>MHHHHHHAAGIPMNNPAIKRIGNHITKSPEDKREYRGLELANGIKVLLISDPTTDKSSAALDVHIGSLSDPPNIAGLSHFLEHMLFLGTKKYPKENEYSQFLSEHAGSSNAFTSGEHTNYYFDVSHEHLEGALDRFAQFFLSPLFDESAKDREVNAVDSEHEKNVMNDAWRLFQLEKATGNPKHPFSKFGTGNKYTLETRPNQEGIDVRQELLKFHSAYYSSNLMAVVVLGRESLDDLTNLVVKLFSEVENKNVPLPEFPEHPFQEEHLKQLYKIVPIKDIRNLYVTFPIPDLQKYYKSNPGHYLGHLIGHEGPGSLLSELKSKGWVNTLVGGQKEGARGFMFFIINVDLTEEGLLHVEDIILHMFQYIQKLRAEGPQEWVFQELKDLNAVAFRFKDKERPRGYTSKIAGILHYYPLEEVLTAEYLLEEFRPDLIEMVLDKLRPENVRVAIVSKSFEGKTDRTEEWYGTQYKQEAIPDEVIKKWQNADLNGKFKLPTKNEFIPTNFEILPLEKEATPYPALIKDTAMSKLWFKQDDKFFLPKANLNFEFFSPFAYVDPLHSNMAYLYLELLKDSLNEYAYAAELAGLSYDLQNTIYGMYLSVKGYNDKQPILLKKIIEKMATFEIDEKRFEIIKEAYMRSLNNFRAEQPHQHAMYYLRLLMTEVAWTKDELKEALDDV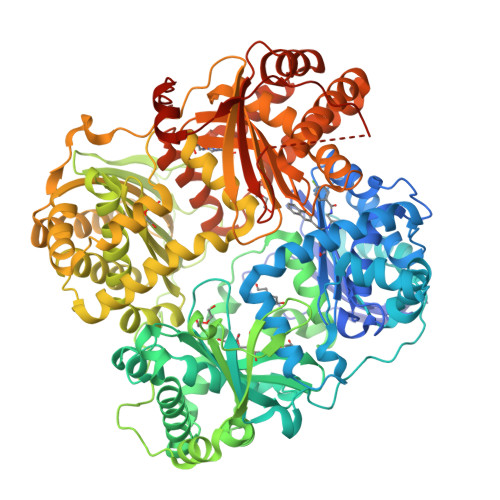TLPRLKAFIPQLLSRLHIEALLHGNITKQAALGIMQMVEDTLIEHAHTKPLLPSQLVRYREVQLPDRGWFVYQQRNEVHNNSGIEIYYQTDMQSTSENMFLELFAQIISEPAFNTLRTKEQLGYIVFSGPRRANGIQGLRFIIQSEKPPHYLESRVEAFLITMEKSIEDMTEEAFQKHIQALAIRRLDKPKKLSAESAKYWGEIISQQYNFDRDNTEVAYLKTLTKEDIIKFYKEMLAVDAPRRHKVSVHVLAREMDSNPVVGEFPAQNDINLSQAPALPQPEVIQNMTEFKRGLPLFPLVKPHINFMAAKL[2x]> GSHMSRLDKSKVINSALELLNE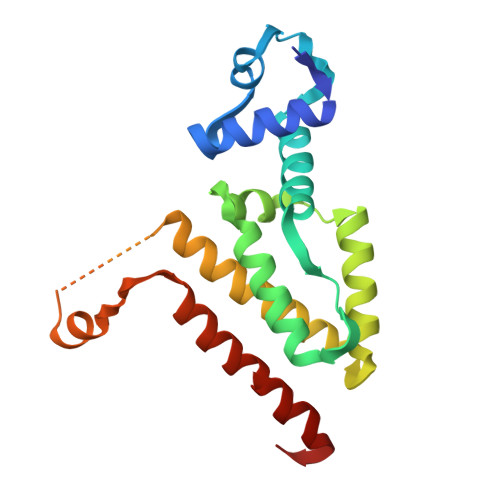VGIEGLTTRKLAQKLGVEQPTLYWHVKNKRALLDALAVEILARHHDYSLPAAGESWQSFLRNNAMSFRRALLRYRDGAKVHLGTRPDEKQYDTVETQLRFMTENGFSLRDGLYAISAVSHATLGAVLEQQEHTAALTDRPAAPDENLPPLLREALQIMDSDDGEQAFLHGLEWLIRGFEVQLTALLQIV>ETDVTSDTVEVLPQHKFDLRSLEAYLNQHLPGFGSDSRAVLTVTQYRSGQSNPTFFLQKGSQAYVLRKKPPGSLLPKAHKIDREFKIQKALFSIGFPVAKPLLYCRDASVIGTEFYVMEHVQGRIFRDFSIPGVSSAERAAIYVSVAETLAWLHSLDIRSLKLDKYGTGVGYCKRQVSTWTKQYQASAHQSIPAMDQLSTWLMKNLPDSDSEECLVHGDFKLDNIVFHPKECRVIAVLDWELSTFGHPLTDLAHLSLFYYWPRTLPMINRGSHIPENTGIPLMEELISIYCHRRGIDPNLPNWNFFMALSFFKLAGISQGVYRRYLMGNNSSEDSFLTANTVQPLAETGLQLSKRTLRTTPPQADAKSQLFAQSRRGQEVLTRVKQFMKQHVFPAEKEVAEYYAQSGNSAEKWGHPLVIEKLKEIAKAEGLWNLFLPAVSGLSQVDYALIAEETGKCFFAPDVFNCQAPDTGNMEVLHLYGSEQQKKQWLEPLLRGDITSVFCMTEPNVSSSDATNIECTIQRDGGGYIVNGKKWWSSGAGNPKCKIAIVLGRTESPSASRHRQHSMILVPMDTPGVELIRPLSVFGYMDNMHGGHWEVHFNHVRVPASNLILGEGRGFEISQGRLGPGRIHHCMRTVGLAERILQIMCDRAVQREAFKKKLYEHEVVAHWIAKSRIAIEEIRLLTLKAAHSIDTLGSASARKEIAMIKVAAPKAVCKIADWAIQVHGGAGVSQDYPLANMYAIIRTLRLANGPDEVHLSAIAKMELQDQARRLTARM[4x]

Here we reveal that two atypical acyl-CoA dehydrogenases, ACAD10 and ACAD11, drive 4-HA catabolism in mice. Unlike other ACADs, ACAD10 and ACAD11 feature kinase domains that phosphorylate the 4-hydroxy position as a requisite step in converting 4-hydroxyacyl-CoAs into conventional 2-enoyl-CoAs. ACAD10/11 are evolutionarily divergent members of the ACAD family, possessing both an N-terminal kinase domain and unconventional hydrophilic residues in the ACAD active site. These features allow them to phosphorylate and process 4-hydroxylated acyl-CoA substrates, ultimately removing the hydroxy group and producing 2-enoyl-CoAs that can enter the FAO cycle.

In the second mutant (A*), we replaced the catalytic aspartate of the ACAD domain with asparagine, eliminating the ACAD activity but leaving kinase activity intact. To further explore the bifunctionality of ACAD10/11 at the molecular level, we initiated cryo-electron microscopy (cryo-EM) experiments with the ACAD11 K* and A* mutant proteins purified from Escherichia coli. To assess whether substrate interactions affect protein structure, these mutants were incubated with 4-HV-CoA and 4-PV-CoA, respectively, before preparation. a, Cryo-EM map and model of the ACAD11 A* mutant tetramer incubated with 4-PV-CoA. The active sites of the tetrameric ACAD domain show density that is consistent with bound flavin adenine dinucleotide (FAD). R626, H634 and R637 are found on a single α-helix within the ACAD domain active site that is directly adjacent to the catalytic D753. To understand how these residues may interact with the 4-phosphoacyl-CoA substrate, we modeled 4-phospho-octanoyl-CoA into the ACAD11 A* ACAD domain. The 4-phospho group is directly stabilized by salt bridges with H634, R637 and R626—residues not found in conventional ACADs—while the hydrophobic tail itself extends toward a broad but closed cavity with a largely hydrophobic surface, suggesting the domain can accommodate much longer substrates. To explore how the kinase domain might bind an acyl-CoA substrate, we modeled 4-hydroxyoctanoyl-CoA (4-HO-CoA) in the ACAD11 A* kinase domain’s active site pocket. We observed that a substantial portion of the CoA moiety associated with residues inside a cavity adjacent to the active site opening.(pyridin-2-ylmethyl)phosphonic acid | C6 H8 N O3 P | 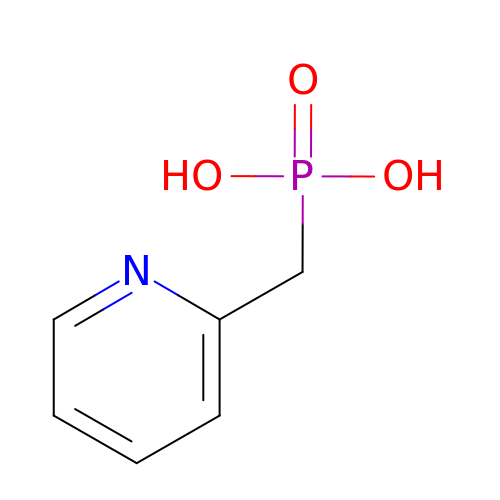WVWCWWLEFNGDBC-UHFFFAOYSA-N> GNQPSTSARARLIDPGFGIYKVNELVDARDVGLGAWFEAHIHSVTRASDGQSRGKTPLKNGNIKHKSKENTNKLDSVPSTSNSDCVAADEDVIYHIQYDEYPESGTLEMNVKDLRPRARTILKWNELNVGDVVMVNYNVESPGQRGFWFDAEITTLKTISRTKKELRVKIFLGGSEGTLNDCKIISVDEIFKIERPGAHPLSFADGKFLRRNDPECDLCGGDPEKKCHSCSCRVCGGKHEPNMQLLCDECNVAYHIYCLNP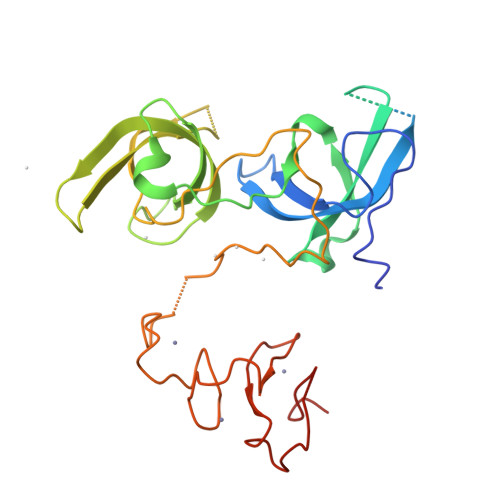PLDKVPAEEYWYCPSCKTD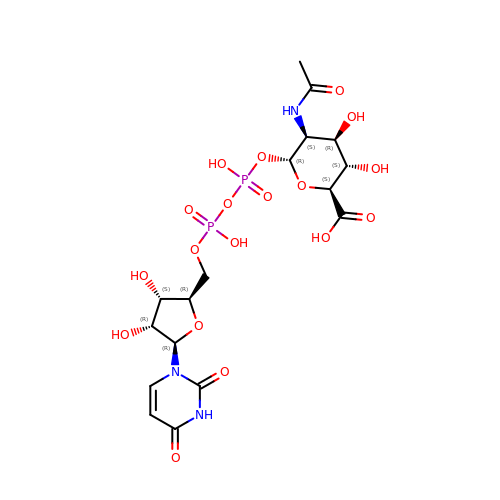(2S,3S,4R,5S,6R)-5-acetamido-6-[[[(2R,3S,4R,5R)-5-[2,4-bis(oxidanylidene)pyrimidin-1-yl]-3,4-bis(oxidanyl)oxolan-2-yl]methoxy-oxidanyl-phosphoryl]oxy-oxidanyl-phosphoryl]oxy-3,4-bis(oxidanyl)oxane-2-carboxylic acid | C17 H25 N3 O18 P2 | DZOGQXKQLXAPND-XHUKORKBSA-N> QNNVPNTFTDPDSGITFNTWGLDEDSPQTQGGFTFGVALPSDALTTDASEFIGYLKCARNDESGWCGISLGGPMTNSLLITAWPHEDTVYTSLRFATGYAMPDVYEGDAEITQVSSSVNSTHFSLIFRCKNCLQWSHGGSSGGASTSGGVLVLGWVQAFDDPGNPTCPEQITLQQHDNGMGIWGAQLNTDAASPSYTDWAAQATKTVTGDCEGPTETSVVGVPVPTGVSFDYIVVGGGAGGIPAADKLSEAGKSVLLIEKGFASTANTGGTLGPEWLEGHDLTRFDVPGLCNQIWVDSKGIACEDTDQMAGCVLGGGTAVNAGLWFKPYSLDWDYLFPDGWKYNDVQPAINRALSRIPGTDAPSTDGKRYYQEGFEVLSKGLAAGGWTSVTANN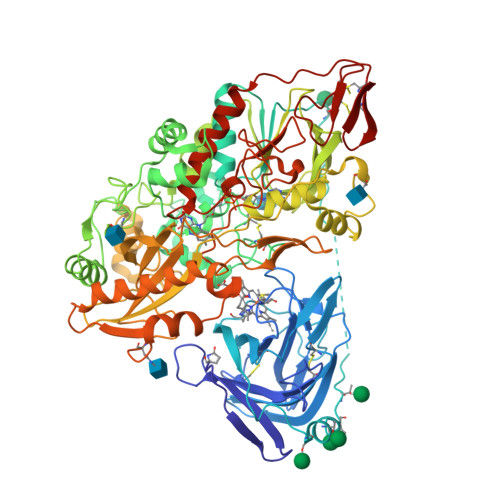APDKKNRTFAHAPFMFAGGERNGPLGTYFQTAKKRNNFDVWLNTSVKRVIREGGHITGVEVEPFRDGGYEGIVPVTKVTGRVILSAGTFGSAKILLRSGIGPEDQLEVVAASEKDGPTMIGNSSWINLPVGYNLDDHLNTDTVISHPDVVFYDFYEAWDDPIESDKNSYLESRTGILAQAAPNIGPMFWEEIVGADGIVRQLQWTARVEGSLGAPNGHTMTMSQYLGRGATSRGRMTITPSLTTIVSDVPYLKDPNDKEAVIQGIINLQNALQNVANLTWLFPNSTITPREYVESMVVSPSNRRSNHWMGTNKLGTDDGRKGGSAVVDLDTRVYGTDNLFVIDASIFPGVPTTNPTSYIVVAAEHASSRILALPDLEPVPKYGQCGGREWTGSFVCADGSTCEYQNEWYSQCL>MDLATLLGLIGGFAFVIMAMVLGGSIGMFVDVTSILIVVGGSIFVVLMKFTMGQFFGATKIAGKAFMFKADEPEDLIAKIVEMADAARKGGFLALEEMEINNTFMQKGIDLLVDGHDADVVRAALKKDIALTDERHTQGTGVFRAFGDVAPAMGMIGTLVGLVAMLSNMDDPKAIGPAMAVALLTTLYGAILSNMVFFPIADKLSLRRDQETLNRRLIMDGVLAIQDGQNPRVIDSYLKNYLNEGKRALEIDE[5x];>MDDEDNKCDCPPPGLPLWMGTFADLMSLLMCFFVLLLSFSEMDVLKFKQIAGSMKFAFGVQNQLEVKDIPKGTSIIAQEFRPGRPEPTPIDVIMQQTMDITQQTLEFHEGESERAGGTKRDEGKLTGGQSPETSTQNNESAEADMQQQQSKEMSQEMETLMESIKKALEREIEQGAIEVENLGQQIVIRMREKGAFPEGSAFLQPKFRPLVRQIAELVKDVPGIVR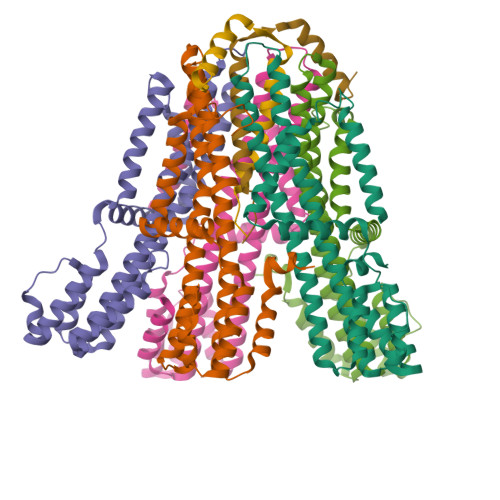VSGHTDNRPLDSELYRSNWDLSSQRAVSVAQEMEKVRGFSHQRLRVRGMADTEPLLPNDSDENRALNRRVEISIMQGEPLYSEEVPVIQ[2x]>MGSSHHHHHHGSTKYALVGDVGGTNARLALCDIASGEISQAKTYSGLDYPSLEAVIRVYLEEHKVEVKDGCIAIACPITGDWVAMTNHTWAFSIAEMKKNLGFSHLEIINDFTAVSMAIPMLKKEHLIQFGGAEPVEGKPIAVYGAGTGLGVAH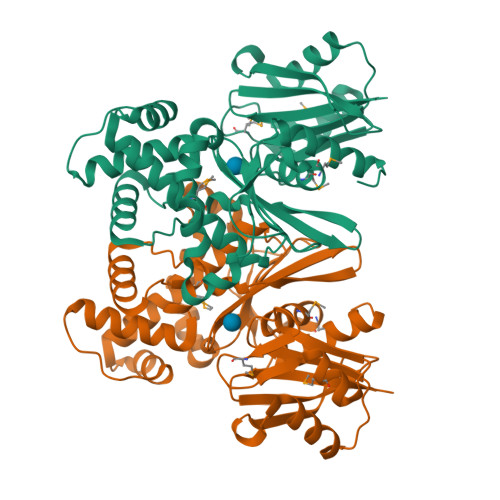LVHVDKRWVSLPGEGGHVDFAPNSEEEAIILEILRAEIGHVSAERVLSGPGLVNLYRAIVKADNRLPENLKPKDITERALADSCTDCRRALSLFCVIMGRFGGNLALNLGTFGGVFIAGGIVPRFLEFFKASGFRAAFEDKGRFKEYVHDIPVYLIVHDNPGLLGSGAHLRQTLGHIL[2x]> VEFNTDVLDAADKKNIDFTRFSEAGYVLPGQYLLDVIVNGQSISPASLQISFVEPQSSGDKAEKKLPQACLTSDMVRLMGLTAESLDKVVYWHDGQCADFHGLPGVDIRPDTGAGVLRINMPQARLEYSDATWLPPSRWDDGIPGLMLDYNLNGTVSRNYQGGDSHQFSYNGTVGGNLGPWRLRADYQGSQEQSRYNGEKTTNRNFTWSRFYLFRAIPRWRANLTLGENNINSDIFRSWSYTGASLESDDRMLPPRLRGYAPQITGIAETNARVVVSQQGRVLYDSMVPAGPFSIQDLDSSVRGRLDVEVIEQNGRKKTFQVDTASVPYLTRPGQVRYKLVSGRSRGYGHETEGPVFATGEASWGLSNQWSLYGGAVLAGDYNALAAGAGWDLGVPGTLSADITQSVARIEGERTFQGKSWRLSYSKRFDNADADITFAGYRFSERNYMTMEQYLNARYRNDYSSREKEMYTVTLNKNVADWNTSFNLQYSRQTYWDIRKTDYYTVSVNRYFNVFGLQGVAVGLSASRSKYLGRDNDSAYLRISVPLGTGTASYSGSMSNDRYVNMAGYTDTFNDGLDSYSLNAGLNSGGGLTSQRQINAYYSHRSPLANLSANIASLQKGYTSFGVSASGGATITGKD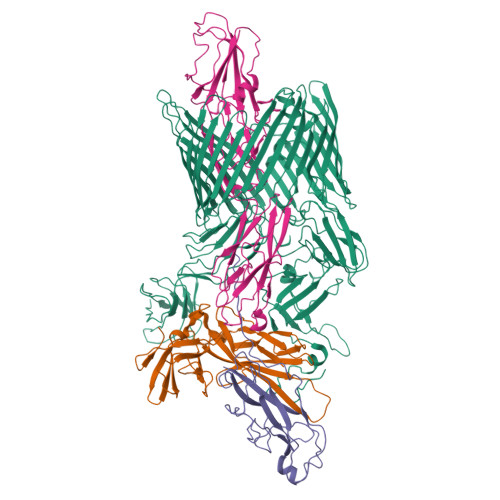AALHAGGMSGGTRLLVDTDGVGGVPVDGGQVVTNRWGTGVVTDISSYYRNTTSVDLKRLPDDVEATRSVVESALTEGAIGYRKFSVLKGKRLFAILRLADGSQPPFGASVTSEKGRELGMVADEGLAWLSGVTPGETLSVNWDGKIQCQVNVPETAISDQQLLLPCTPQK;> MIRKKILMAAIPLFVISGADAAVSLDRTRAVFDGSEKSMTLDISNDNKQLPYLAQAWIENENQEKIITGPVIATPPVQRLEPGAKSMVRLSTTPDISKLPQDRESLFYFNLREIPPRSEKANVLQIALQTKIKLFYRPAAIKTRPNEVWQDQLILNKVSGGYRIENPTPYYVTVIGLGGSEKQAEEGEFETVMLSPRSEQTVKSANYNTPYLSYINDYGGRPVLSFICNGSRCSVKKEK;> MKKWFPALLFSLCVSGESSAWNNIVFYSLGDVNSYQGGNVVITQRPQFITSWRPGIATVTWNQCNGPGFADGFWAYYREYIAWVVFPKKVMTQNGYPLFIEVHNKGSWSEENTGDNDSYFFLKGYKWDERAFDAGNLCQKPGETTRLTEKFDDIIFKVALPADLPLGDYSVKIPYTSGMQRHFASYLGARFKIPYNVAKTLPRENEMLFLFKNIGGCRPSAQSLEIKHGDLSINSANNHYAAQTLSVSCDVPANIRFMLLRNTTPTYSHGKKFSVGLGHGWDSIVSVNGVDTGETTMRWYKAGTQNLTIGSRLYGESSKIQPGVLSGSATLLMILP;> MIKSTGALLLFAALSAGQAIASDVAFRGNLLDRPCHVSGDSLNKHVVFKTRASRDFWYPPGRSPTESFVIRLENCHATAVGKIVTLTFKGTEEAALPGHLKVTGVNAGRLGIALLDTDGSSLLKPGTSHNKGQGEKVTGNSLELPFGAYVVATPEALRTKSVVPGDYEATATFELTYR> MIIPALNLIDGTVVRLHQGDYARQRDYGNDP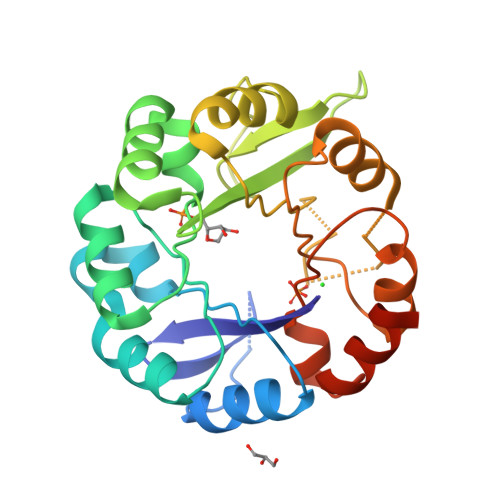LPRLQDYAAQGAGVLHLVDLTGAKDPAKRQIPLIKTLVAGVNVPVQVGGGVRTEEDVAALLKAGVARVVIGSTAVKSPDVVKGWFERFGAQALVLALDVRIDEHGTKQVAVSGWQENSGVSLEQLVETYLPVGLKHVLCTDISRDGTLAGSNVSLYEEVCARYPQIAFQSSGGIGDIDDIAALRGTGVRGVIVGRALLEGKFTVKEAIQCWQNVKGHHHHHH Dinucleases of the DEDD superfamily, such as oligoribonuclease, Rexo2 and nanoRNase C, catalyze the essential final step of RNA degradation, the conversion of di- to mononucleotides. The active sites of these enzymes are optimized for substrates that are two nucleotides long, and do not discriminate between RNA and DNA. The active sites invariably consist of (i) a catalytic DEDDh/y-containing core for divalent cation coordination and catalysis, (ii) a leucine residue that wedges between the two bases of the substrates and (iii) a 5′-phosphate cap that coordinates the 5′ phosphate of the dinucleotides. Here, we identified a novel DEDD subfamily, members of which function as dedicated deoxydinucleases (diDNases) that specifically hydrolyze single-stranded DNA dinucleotides in a sequence-independent manner.

To understand the molecular basis for the specificity of dimeric NrnC homologs toward DNA substrates, we determined a set of crystal structures of diDNases: (i) a complex of diDNaseNoc with dpGG to 1.55 Å and (ii) diDNase from Rhodococcus (diDNaseRho) in its apo state (1.72 Å resolution) and in complex with dpGG (2 Å resolution). Notably, the structure of the apo-form of diDNaseRho resulted from crystals set up in the presence of the RNA substrate pGG. However, no electron density was observed for pGG, confirming the low affinity of the protein for RNA substrates. The biologically relevant assembly in all crystal structures was determined to be a dimer using the ePISA server, which was consistent with the oligomeric state of the proteins in solution. A comparison of structures of apo- and dpGG-bound diDNaseRho revealed no major conformational changes in the protein upon substrate binding (RMSD value of 0.45 Å for 1604 main-chain atoms of a diDNase dimer). However, two minor differences were observed. First, region 142KTPRLS147 appeared disordered in the apo structure of diDNaseRho, but became visible and folded into a small helix when the substrate was present, owing to the direct interactions of the region with dpGG. Second, three side chains coordinating the substrate, H88, H89, and Y213, adopt different rotamer conformations and turn toward the substrate in diDNaseRho-dpGG.

> SMKKIDPLASTVVVRDGDLSSSFLAAARQCGRVTIDTETTGLSPKIDGLCTVQLHVPGVGTEIVRVDPTLQPTRLLQVLAAEEIVKGFHHAVFDLGFLRHTFQSKARSVVCSKVAAKILWPHDKDRQSLAGLAHLLLGVVLDKTPRLSDWSQPELTKTQVHYAAVDVEILPPILDELDRLLSERQLRELAVACWHHIPAHVELLEHNLGDVFTY> ASPSSELRRALEANEFIPYYQPLSPGQGGRWIGVEVLMRWRHPREGLIRPDLFIPFAERSGLIVPMTRALMRQVAEDLGGHAGKLEPGFHIGFNISATHCHELALVDDCRELLAAFPPGHITLVLELTERELIESSEVTDRLFDELHALGVKI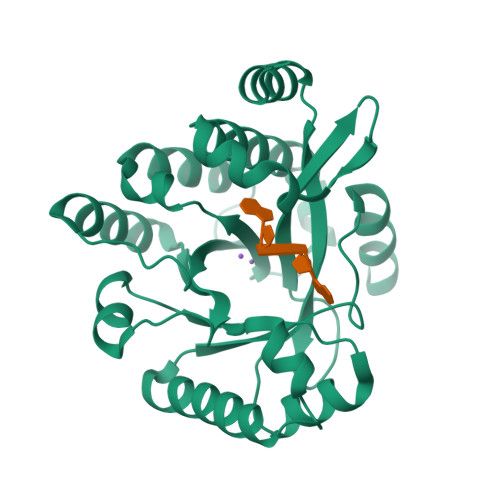AIDDFGTGHSSLAYLRKFQVDCLKIDQSFVARIGIDTLSGHILDSIVELSAKLDLDIVAEGVETPEQRDYLAARGVDYLQGYLIGRPMPLESLLSSLTVQE> MEYQHWLREAISQLQASESPRRDAEILLEHVTGRGRTFILAFGETQLTDEQCQQLDALLTRRRDGEPIAHLTGVREFWSLPLFVSPATLIPRPDTECLVEQALARLPEQPCRILDLGTGTGAIALALASERPDCEIIAVDRMPDAVSLAQRNAQHLAIKNIHILQSDWFSALAGQQFAMIVSNPPYIDEQDPHLQQGDVRFEPLTALVAADSGMADIVHIIEQSRNALVSGGFLLLEHGWQQGEAVRQAFILAGYHDVETCRDYGDNERVTLGRYY;> MKPSIVAKLEALHERHEEVQALLGDAQTIADQERFRALSREYAQLSDVSRCFTDWQQVQEDIETAQMMLDDPEMREMAQDELREAKEKSEQLEQQLQVLLLPKDPDDERNAFLEVRAGTGGDEAALFAGDLFRMYSRYAEARRWRVEIMSASEGEHGGYKEIIAKISGDGVYGRLKFESGGHRVQRVPATESQGRIHTSACTVAVMPELPDAELPDVNPADLRIDTFRSSGAGGQHVNTTDSAIRITHLPTGIVVECQDERSQHKNKAKALSVLGARIHAAEMAKRQQAEASTRRNLLGSGDRSDRNRTYNFPQGRV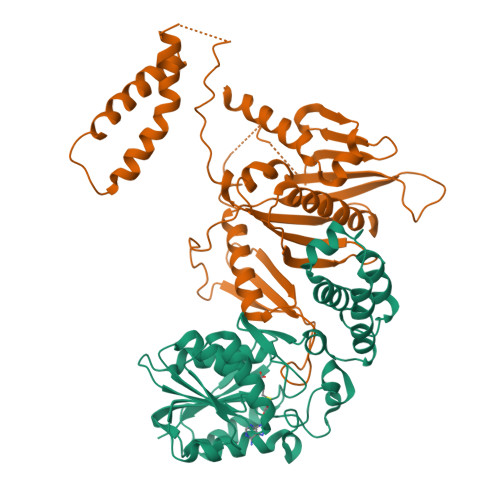TDHRINLTLYRLDEVMEGKLDMLIEPIIQEHQADQLAALSEQE>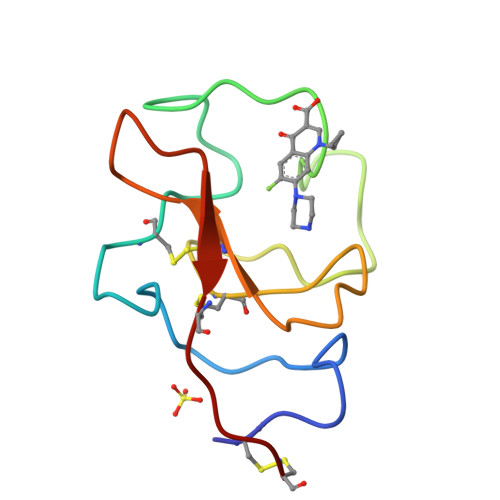 DCMFGNGKGYRGKKATTVTGTPCQEWAAQEPHRHSTFIPGTNKWAGLEKNYCRNPDGDINGPWCYTMNPRKLFDYCDIPLC>MQLNVRSTASGARSSTRSRRMTAVVQAVAQRAGTIDVQRNENFGKLRAGYLFPEIARRRKAHQEKNPDAKIISLGIGDTTEPLPKYIADAMAKAAAGLATREGYSGYGAEQGQGALREAVASTFYGHAGRAADEIFISDGSKCDIARIQMMFGSKPTVAVQDPSYPVYVDTSVMMGMTGDHNGTGFDGIEYMVCNPDNHFFPDLSKAKRTDIIFFCSPNNPTGAAATRAQLTELVNFARKNGSILVYDAAYALYISNPDCPKTIYEIPGADEVAIETCSFSKYAGFTGVRLGWTVVPKALKYANGEPVHADWNRVMTTCFNGASNIVQAGGLACLQPEGLKEMNAMIKFYKENAQILKTTFTEMGFSVYGGDDAPYIWVGFPGKPSWDVFAEILERCNIVTTPGSGYGPAGEGFVRASAFGSRENILEAVRRFKEAY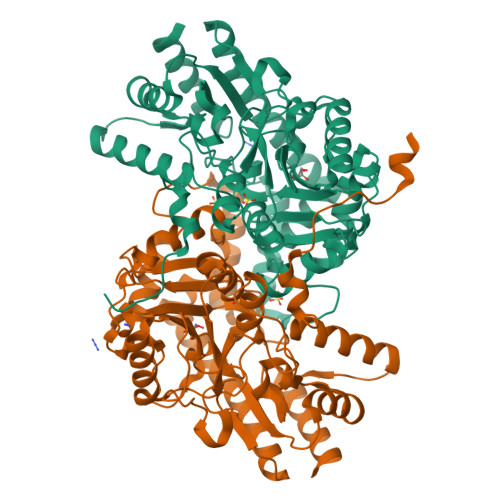GKRNASHHHHHH[2x]> MAHHHHHHSSGQFREFSIETIRNATSGFAAENIVS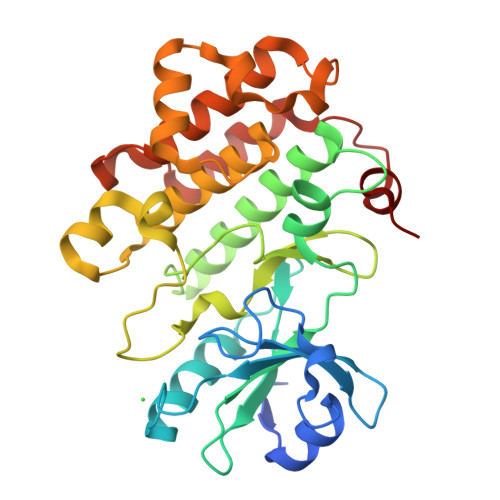EHGERAPNVVYKGKLENQRRIAVKRFNRKSWPDSRQFLEEAKAVGQLRNHRMANLLGCCYEDEERLLIAEFMPNETLAKHLFHWESQPMKWAMRLRVALHIAQALEYCTSKGRALYHDLNAYRVLFDDDANPRLSCFGLMKNSRDGKSYSTNLAFTPPEYLRTGRVTPESVIYSFGTLLLDLLSGKHIPPSHALDLIRDRNIQMLMDSGLEGQFSSDDGTELIRLASRCLQYEPRERPNPKSLVSAMIPLQKDLEIASHQLLGVP> AQQAEWRSWEVNKRLEYSLVKGITEFIEQDTEEARQQATRPCEVIEGPLMDGMNVVGDLFGEGKMFLPQVVKSARVMKQAVAYLEPFIEASKEQCKTNGKMVIATVKGDVHDIGKNIVGVVLQCNNYEIVDLGVMVPAEKILRTAKEVNADLIGLSGLITPSLDEMVNVAKEMERQGFTIPLLIGGATTSKAHTAVKIEQNYSGPTVYVQNASRTVGVVAALLSDTQRDDFVARTRKEYETVRIQHGRKKPRTPPVTLEAARDNDFAFDWQAYTPPVAHRLGVQEVEASIETLRNYIDWTPFFMTWSLAGKYPRILEDEVVGVEAQRLFKDANDMLDKLSAEKTLNPRGVVGLFPANRVGDDIEIYRDETRTHVINVSHHLRQQTEKT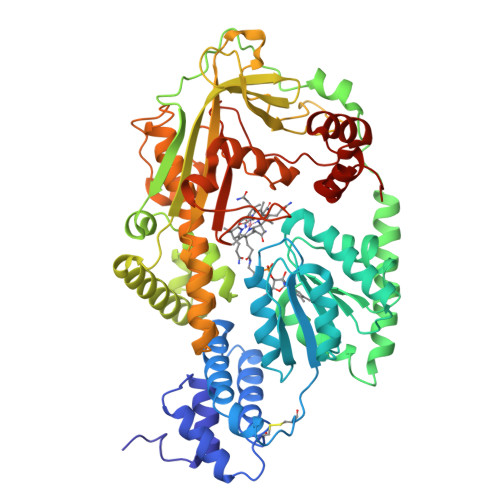GFANYCLADFVAPKLSGKADYIGAFAVTGGLEEDALADAFEAQHDDYNKIMVKALADRLAEAFAEYLHERVRKVYWGYAPNENLSNEELIRENYQGIRPAPGYPACPEHTEKATIWELLEVEKHTGMKLTESFAMWPGASVSGWYFSHPDSKYYAVAQIQRDQVEDYARRKGMSVTEVERWLAPNLGYDAD> GSGGSGGITEAQARAIVNSALKLYSQDKTGMVDFALESGGGSILSTRCSETYETKTALMSLFGIPLWYFSQSPRVVIQPDIYPGNCWAFKGSQGYLVVRLSMMIHPAAFTLEHIPKTLSPTGNISSAPKDFAVYGLENEYQEEGQLLGQFTYDQDGESLQMFQALKRPDDTAFQIVELRIFSNWGHPEYTCLYRFRVHGEPVK;> GSMTSGTSGTSGGPSPPPTWPHLQLCYLQ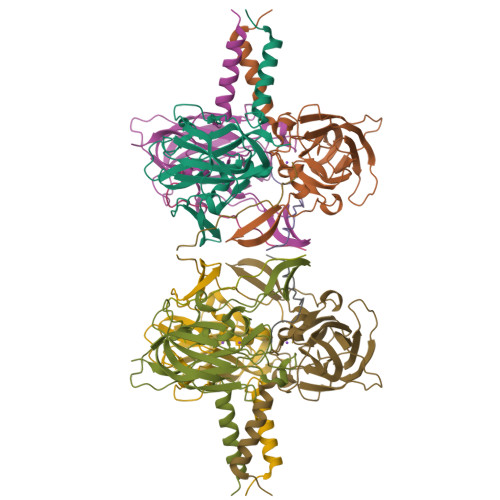PPPV> MVMKLYYFPGACSLAPHIVLR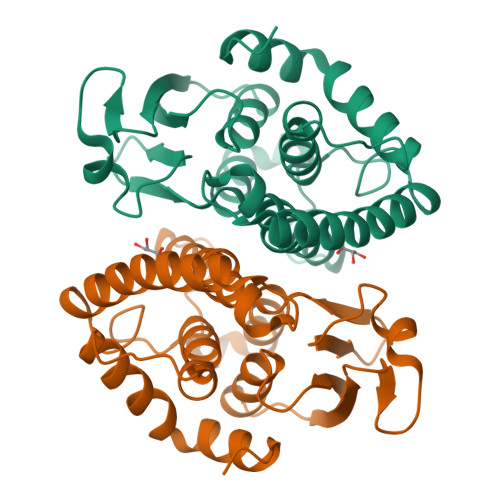EAGLDFELENVDLGTKKTGSGADFLQVNPKGYVPALQLDDGQVLTEDQVILQYLADLKPESGLMPPSGTFERYRLLEWLAFISTEIHKTFGPFWNPESPEASKQIALGLLSRRLDYVEDRLEAGGPWLMGDRYSVADAYLSTVLGWCEYLKIDLSKWPRILAYLERNQARPAVQAAMKAEGLIQAENLYFQSHHHHHHWSHPQFEK DENDRON D2-1 | C49 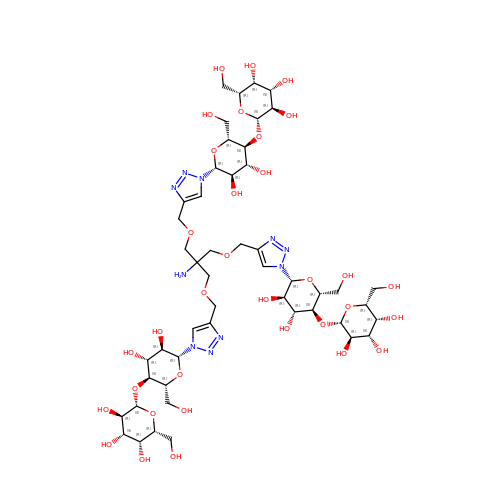H80 N10 O33 | SJELSRWZDPHJDW-KWHDUCOQSA-N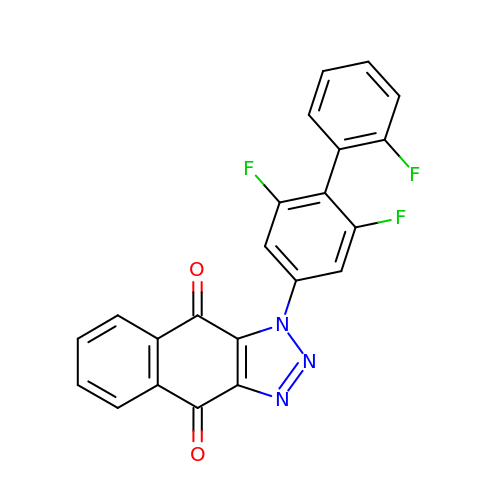3-[3,5-bis(fluoranyl)-4-(2-fluorophenyl)phenyl]benzo[f]benzotriazole-4,9-dione | C22 H10 F3 N3 O2 | VMUZFSZBQDZDTG-UHFFFAOYSA-N> GSHMHESKEWYHASLTRAQAEHMLMRVPRDGAFLVRKRNEPNSYAISFRAEGKIKHCRVQQEGQTVMLGNSEFDS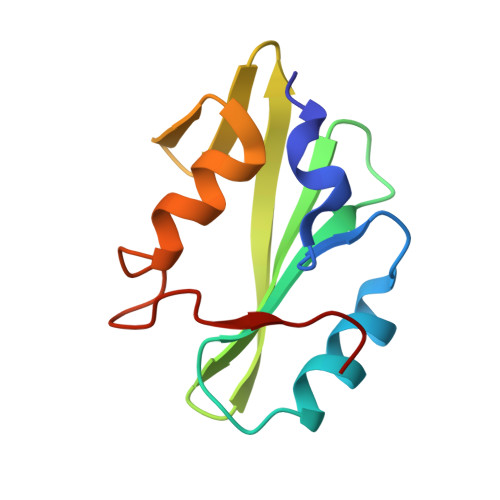LVDLISYYEKHPLYRKMKLRYPINEE> AMADTIVAVELDSYPNTDIGDPSYPHIGIDIKSIRSKSTARWNMQTGKVGTAHISYNSVAKRLSAVVSYSGTSSTTVSYDVDLNNVLPEWVRVGLSATTGLYKETNTILSWSFTS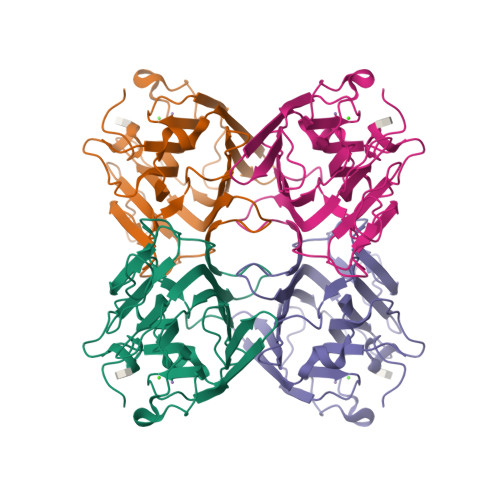KLKTNSIADANSLHFSFHQFSQNPKDLILQSDATTDSDGNLQLTRVSSDGSPQGSSVGRALFYAPVHIWEKSAVVASFDATFTFLIKSPDRDPADGITFFIANTDTSIPSGSGGRLLGLFPDAN> QECTKFKVSSCRECIESGPGCTWCQKLNFTGPGDPDSIRCDTRPQLLMRGCAADDIMDPTSLAETQEDHNGGQKQLSPQKVTLYLRPGQAAAFNVTFRRAKGYPIDLYYLMDLSYSMLDDLRNVKKLGGDLLRALNEITESGRIGFGSFVDKTVLPFVNTHPDKLRNPCPNKEKECQPPFAFRHVLKLTNNSNQFQTEVGKQLISGNLDAPEGGLDAMMQVAACPEEIGWRNVTRLLVFATDDGFHFAGDGKLGAILTPNDGRCHLEDNLYKRSNEFDYPSVGQLAHKLAENNIQPIFAVTSRMVKTYEKLTEIIPKSAVGELSEDSSNVVQLIKNAYNKLSSRVFLDHNALPDTLKVTYDSFCSNGVTHRNQPRGDCDGVQINVPITFQVKVTATECIQEQSFVIRALGFTDIVTVQVLPQCECRCRDQSRDRSLCHGKGFLECGICRCDTGYIGKNCECQTQGRSSQELEGSCRKDNNSIICSGLGDCVCGQC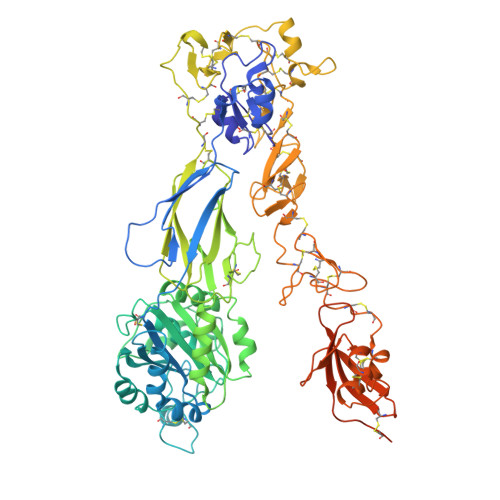LCHTSDVPGKLIYGQYCECDTINCERYNGQVCGGPGRGLCFCGKCRCHPGFEGSACQCERTTEGCLNPRRVECSGRGRCRCNVCECHSGYQLPLCQECPGCPSPCGKYISCAECLKFEKGPFGKNCSAACPGLQLSNNPVKGRTCKERDSEGCWVAYTLEQQDGMDRYLIYVDESRECVDGCGLENLYFQGGKNAQCKKKLQALKKKNAQLKWKLQALKKKLAQGGHHHHHH>SNAMDSRFLPATAFIDPEGRNRNEVERLVQQVVDLILAKLTGAAERPPMPETVDLPGPITIPEAAATEATLLQAIRDMVDGSMNPANPGYIGHMDPMPATMAILGDLVAAAVNNNMLSLEMSPSFSRLETLLLRAIAGLFGLGEQAGGVLTSGGSLANLQALAVARNVAFDSVEPGITGLAQRPVIFASEAAHTSLQKAAMLLGLGTAAVIPVRATADSRMDPEDLRARIDQARGAGQHPFCVVATAGTTTTGNIDPLAEIGAIAREHGLWFHVDAAYGGALVFSERHRWRLAGIEQADSITFNPQKW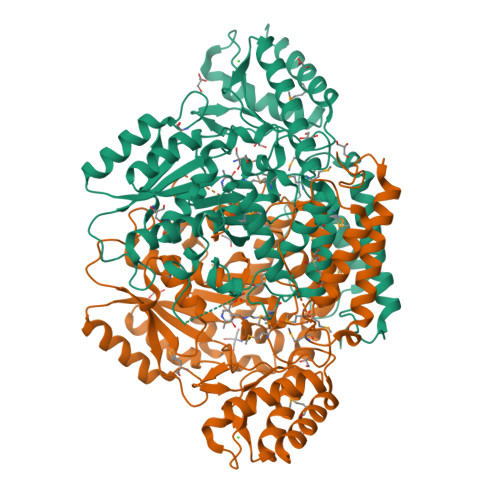LYVAKTCAMVLFRDAGVLERAFRIPAPYMRATDGFINLGEIGVQGTRHADVVKLWLTLQHIGQQGYARLIDDGYRLAERVVEGVRQRPFLRLAGEIDTNIVCFRGEPDWLPAERWDDWNAALQALLLREGKIFLSLPVYRGGRWLRAVLLNPYTTDAVIDAMFKQIDRFAGRERGQER[2x]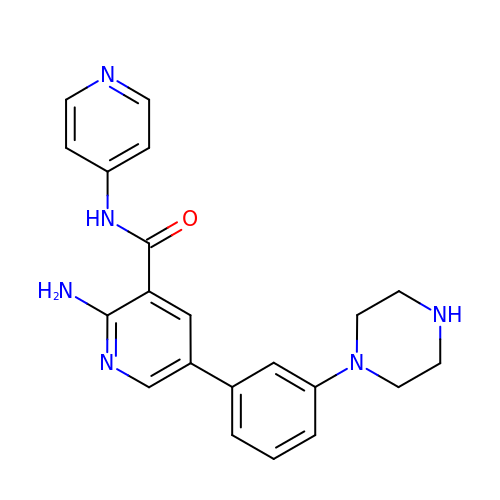2-amino-5-[3-(piperazin-1-yl)phenyl]-N-(pyridin-4-yl)pyridine-3-carboxamide | C21 H22 N6 O | YDMJAALVMGFGRY-UHFFFAOYSA-N>QCVKLNDGHFMPVLGFGTYAPPEVPRSKALEVTKLAIEAGFRHIDSAHLYNNEEQVGLAIRSKIADGSVKREDIFYTSKLWSTFHRPELVRPALENSLKKAQLDYVDLYLIHSPMSLKPGEELSPTDENGKVIFDIVDLCTTWEAMEKCKDAGLAKSIGVSNFNRRQLEMILNKPGLKYKPVCNQVECHPYFNRSKLLDFCKSKDIVLVAYSALGSQRDKRWVDPNSPVLLEDPVLCALAKKHKRTPALIALRYQLQRGVVVLAKSYNEQRIRQNVQVFEFQLTAEDMKA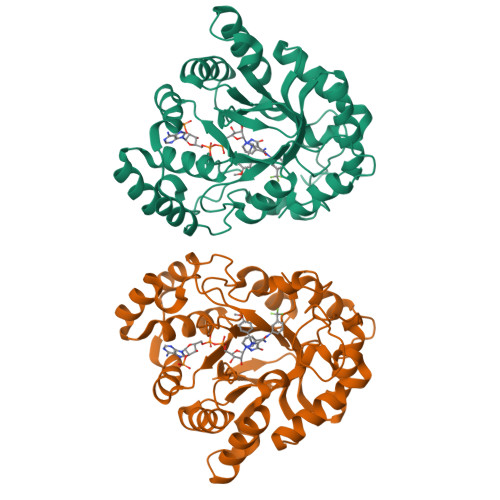IDGLDRNLHYFNSDSFASHPNYPY[2x]> GPGSTQYNFIIDASAFEKGLGNIKRWCSDCTEAVTLNFYIPTFTLNELDFLQQRRKSFAARESLKFIDRLDDSKFANLKVFIEFPEVLDIILWSDVMEHNDSSGKINIAKLPKRLKNLLKSCIYKCYLEGNEGLHWFLISEDPQIREMAMQCNIPSCSIVDVDSILSKDM

Among these, the nonsense-mediated mRNA decay (NMD) pathway is responsible for the rapid detection and degradation of translated mRNAs harboring premature termination codons (PTCs), which can arise from mutations, transcription, or processing errors as well as alternative or defective splicing events. UPF1 is made of 2 structured domains: a CH-domain known to interact with UPF2 and an ATP-dependent RNA helicase domain (HD). Nmd4 is composed of a PIN domain (for PilT N-terminus) and interacts directly with the helicase domain of Upf1. Nmd4 stimulates Upf1-HD ATPase activity and strengthens Upf1-HD binding to RNA.

We also determined the 1.8 Å resolution crystal structure of the PIN domain of Nmd4 (residues 1 to 167) to help us solve the structure of the Nmd4/Upf1-HD complex. As this structure is virtually identical to the structure of the PIN domain of Nmd4 in the complex (rmsd of 0.5 Å over 163 Cα atoms between the 2 structures), we will only describe the structure of this domain in the Upf1-Nmd4 complex. The Nmd4 protein is composed of 2 domains. First, a PIN domain (residues 1 to 167), which is structurally similar to the PIN domains of Kluyveromyces lactis Nmd4 (KlNmd4; ) and of the human proteins SMG5 and SMG6. As previously observed for KlNmd4, the catalytic residue D1353 of the human SMG6 protein corresponds to a leucine (Leu112) in the S. cerevisiae Nmd4 protein. Since the D1353A mutation completely abolishes the enzymatic activity of SMG6, this strongly suggests that the PIN domain of Nmd4 is not endowed with endonucleolytic activity. This is in line with the lack of evidence for such activity in the yeast NMD pathway, in contrast to what has been shown in metazoans.>GPHMSEAKAKAIGKVDDLLELYMGIRDIDLATTMFEAGKDKSNPDEFAVALDETLGDFAFPDEFLFDVWGAISDMKQGR[5x];>GPGSHDLSKWKYAELRDTINTSCDIELLAACREEFHRRLKVYHAWKSKN[5x]

GIPC1 (GAIP interacting protein, C-terminus 1) and its two paralogs GIPC2 and GIPC3 are universal adaptor proteins that bind and regulate vesicular trafficking of many transmembrane proteins. GIPCs contribute to the endocytosis process by tethering the cargo proteins on endocytic vesicles to the motor protein myosin VI. GIPCs contain a central PDZ (PSD-95, Dlg and ZO-1) domain that mediates the interaction with the C-terminal PDZ-binding motif (PBM) in cargo proteins. The transmembrane receptor PlexinD1 contains a C-terminal ‘SEA’ motif that constitutes a PBM and interacts with GIPC1.

We determined the crystal structures of the myosin VI-HCBD in complex with the GH2 domain from GIPC1 and GIPC2, respectively. The GIPC2-GH2/myosin VI structure forms the same alternating array, despite being crystallized in a different condition and space group. The recurrence of this repeating array argues strongly that this arrangement captures the oligomeric interaction mode between GIPCs and myosin VI that is relevant to function, rather than being a crystal packing artifact. The bivalent interactions between the GIPC-GH2 and myosin VI-HCBD are mediated by two distinct interfaces. Interface I involves the two loops in the GIPC-GH2 domain, one between helices α1 and α2 and the other between helices α3 and α4. These two loops interact with Arg1084 and Arg1085 in the ‘RRL’ motif on one side of the second helix in the myosin VI-HCBD. The two interfaces in the GIPC2-GH2/HCBD complex structure are highly similar to those in the GIPC1-GH2/HCBD complex. The alternative arrays mediated by the bivalent interactions seen here suggest an unanticipated mechanism for high-order oligomerization of the GIPC/myosin VI complex. The linear array of the GIPC/myosin VI complex formed through their mutual bivalent binding provides an elegant mechanism for myosin VI oligomerization.> MKSSHHHHHHENLYFQSNAELQPQFNEFLANIRPTDTQKEDWKSGARTLRERLKNFEPLKEIVVSTFLQGSIRRSTAIRPLGDKRPDVDIVVVTNLDHTRMSPTDAMDLFIPFLEKYYPGKWETQGRSFGITLSYVELDLVITAIPESGAEKSHLEQLYKSESVLTVNSLEEQTDWRLNKSWTPNTGWLSESNSAQVEDAPASEWKAHPLVLPDREKNEWGRTHPLAQIRWTAEKNRLCNGHYINLVRAVKWWRQQNSEDLPKYPKGYPLEHLIGNALDNGTTSMAQGLVQLMDTFLSRW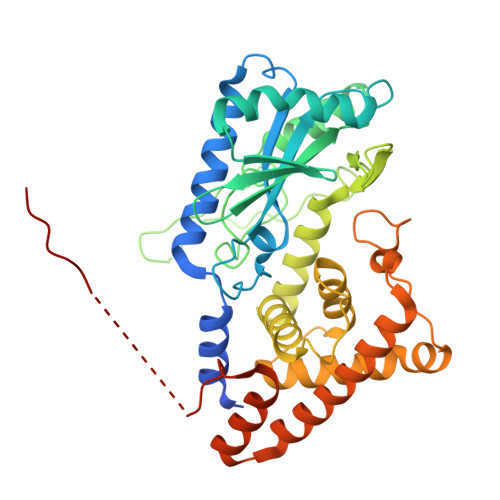AAIYNQKSKPWLSDHGVAEHDVMARLTAEDFCSFYEGIASAAEIARNALASEEPQESAQLWRQLFGSKFPLPGPQGGDRNGGFTTPSKPAEPQKTGRFA>[3x]PATGEKKECWSWESYLEEQKAITAPVSLFQDSQAVTHNKNGFKLGMKLEGIDPQHPSMYFILTVAEVCGYRLRLHFDGYSECHDFWVNANSPDIHPAGWFEKTGHKLQPPKGYKEEEFSWSQYLRSTRAQAAPKHLFVSQSHSPPPLGFQVGMKLEAVDRMNPSLVCVASVTDVV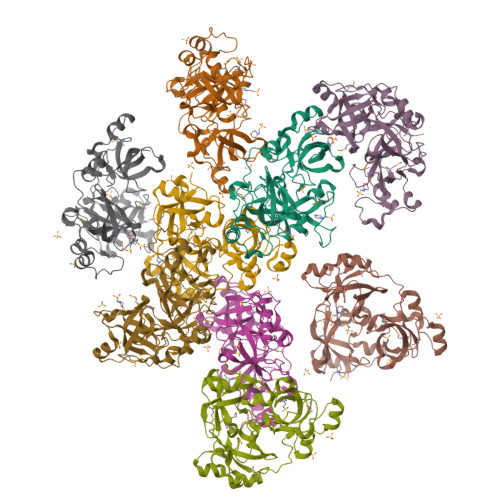DSRFLVHFDNWDDTYDYWCDPSSPYIHPVGWCQKQGKPLTPPQDYPDPDNFCWEKYLEETGASAVPTWAFKVRPPHSFLVNMKLEAVDRRNPALIRVASVEDVEDHRIKIHFDGWSHGYDFWIDADHPDIHPAGWCSKTGHPLQPPLGPREPSSAS>[3x]GSYSHVFTVTVRKATNVTKGAIGDMLDTPDPYVELFIPSAPDCRKRTKHFNNDVNPVWNETFEFILDPNQDNVLEVTLMDANYV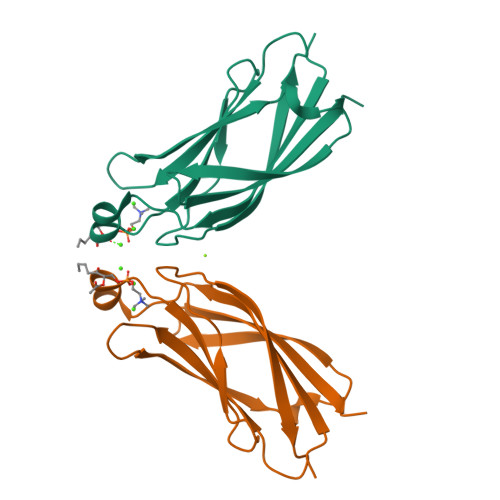MDETLGMATFPISSLKLGEKKEVQLTFNNVTEMTLELSLEVCS cyclohexylmethyl 2-formylphenyl hydrogen (S)-phosphate | C14 H19 O5 P | 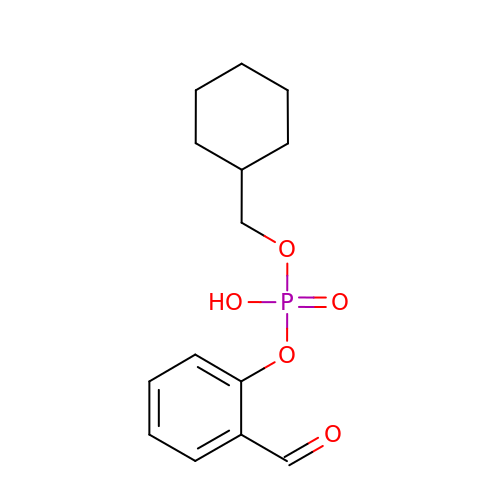YBEVTZVQKMYQPM-UHFFFAOYSA-N> MTDTTNSIKHVISPLARQTLQDRDLTRPVAGKRPIRLLPWLQVVKIGGRVMDRGADAILPLVEELRKLLPEHRLLILTGAGVRARHVFSVGLDLGLPVGSLAPLAASEAGQNGHILAAMLASEGVSYVEHPTVADQLAIHLSATRAVVGSAFPPYHHHEFPGSRIPPHRADTGAFLLADAFGAAGLTIVENVDGIYTADPNGPDRGQARFLPETSATDLAKSEGPLPVDRALLDVMATARHIERVQVVNGLVPGRLTAALRGEHVGTLIRTGVRPA;> MANSTAELEELLMQRSLTDPQLQAAAAAAADFRILPDATVIKIGGQSVIDRGRAAVYPLVDEIVAARKNHKLLIGTGAGTRARHLYSIAAGLGLPAGVLAQLGSSVADQNAAMLGQLLAKHGIPVVGGAGLSAVPLSLAEVNAVVFSGMPPYKLWMRPAAEGVIPPYRTDAGCFLLAEQFGCKQMIFVKDEDGLYTANPKTSKDATFIPRISVDEMKAKGLHDSILEFPVLDLLQSAQHVREVQVVNGLVPGNLTRALAGEHVGTIITAS

As opposed to cryo-crystallography, room-temperature X-ray structures reveal realistic conformational flexibility that is crucial for protein function. The most direct approach is serial millisecond crystallography (SMX), which utilizes the same high-viscosity injectors successful at XFELs to distribute the radiation dose over thousands of crystals to determine room-temperature structures with minimum radiation-damage. To demonstrate the general applicability of SMX, we have chosen three real-life targets: the radiation sensitive molybdenum storage protein (MOSTO), the αβ-tubulin-darpin complex (TD1) soaked with the drug colchicine and the thermostabilised adenosine A2A G protein-coupled receptor (A2AR). In conclusion, we show that SMX at synchrotrons allows fast, straightforward structure determination at room-temperature for large soluble macromolecular complexes as well as membrane proteins.

To examine the time needed to adapt protein crystallization and crystal preparation for SMX, we selected the soluble MOSTO complex whose crystallization was previously optimized for classical crystallography. Room-temperature structure determination of this complex is challenging because of the unusually high metal content, which makes it susceptible to radiation damage. After a simple optimization step, we were able to produce numerous microcrystals suitable for SMX in hanging drops. After embedding these crystals into LCP, we collected 68,788 indexable diffraction patterns in ~6 h with much less time necessary to collect a fully converged data set. The data extended to 1.7 Å resolution, and the resulting electron density map is of excellent quality. Clearly, high-resolution structure determination at room-temperature by SMX can be fast and straightforward. In the case of MOSTO, where we initially suffered from low hit rates, we used a very wide but thin 40 × 5 μm2 beam. In combination with a larger nozzle size, a larger volume could be “scanned”, allowing to collect a large data set within 6 h of beamtime while still obtaining data to high resolution. Based on the average indexing rate, data collection times for these converged data sets were 82, 3 and 10 min for TD1, A2AR SMX and MOSTO, respectively.> MMTMRRHLLLVSNSTLHGGGYLEHCQEHILKFLGAQVKRVLFIPYALHDRDAYAKTARQKFEALGYGLDSVHESPDPVDAVKKAEAIFIGGGNTFRLLKALYDNDLIAAIRKRVLEDGVPYIGSSAGTNVATISINTTNDMPIVYPPSLKALELVPFNINPHYLDPDGNSKHMGETREQRITQYHEEHDTPPVLGLREGCFLLVEGDKATLLGITR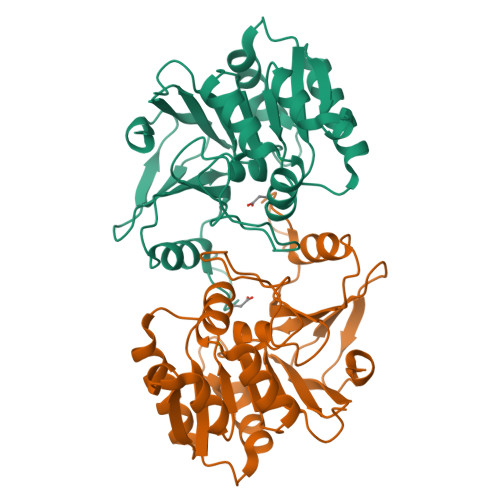ARLFLRGKNPTEHEPGHDFSFLLGHS N-[(2S,4S,5S,7R)-4-AMINO-8-(BUTYLAMINO)-5-HYDROXY-7-METHYL-2-(1-METHYLETHYL)-8-OXOOCTYL]-2-(3-METHOXYPROPOXY)BENZAMIDE | 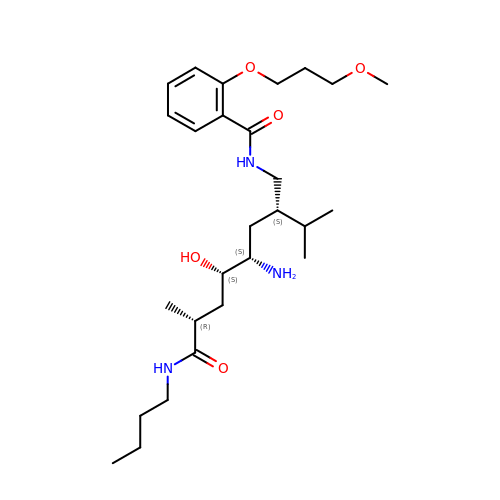C27 H47 N3 O5 | JYPXLSXKONMTFW-HTDNTCHWSA-N>[3x]MPLKPEEHEDILNKLLDPELAQSERTEALQQLRVNYGSFVSEYNDLTKSHEKLAAEKDDLIVSNSKLFRQIGLTDKQEEDHKKADISETITIEDLEAK;> MRITFNDVKTSLGITESYDIVNAIRNSQGDNFKSYVPLATANNVAEVGAGILINQTVQNDFITSLVDRIGLVVIRQVSLNNPLKKFKKGQIPLGRTIEEIYTDITKEKQYDAEEAEQKVFEREMPNVKTLFHERNRQGFYHQTIQDDSLKTAFVSWGNFESFVSSIINAIYNSAEVDEYEYMKLLVDNYYSKGLFTTVKIDEPTSSTGALTEF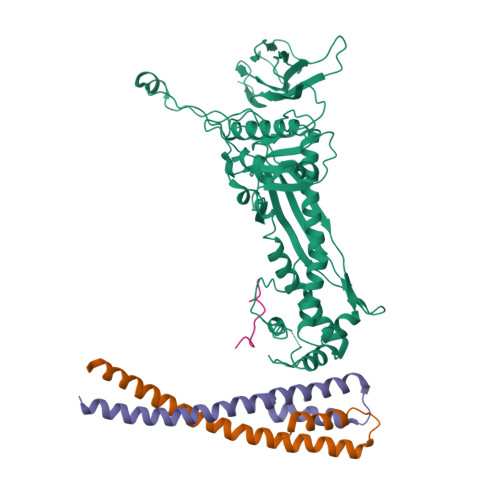VKKMRATARKLTLPQGSRDWNSMAVRTRSYMEDLHLIIDADLEAELDVDVLAKAFNMNRTDFLGNVTVIDGFASTGLEAVLVDKDWFMVYDNLHKMETVRNPRGLYWNYYYHVWQTLSVSRFANAVAFVSGDVPAVTQVIVSPNIAAVKQGGQQQFTAYVRATNAKDHKVVWSVEGGSTGTAITGDGLLSVSGNEDNQLTVKATVDIGTEDKPKLVVGEAVVSIRPNNASGGAQA>MANLNQIQKEVSEI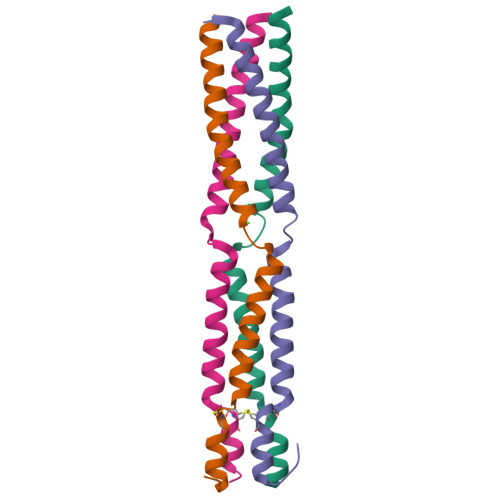LSDQKSMKADIKAILELLGSQNPIKESLETVAAKIVNDLTKLINDCPCNKEILEALGTQPKEQLIEQPKEKGKGLNLGKYS[4x]>[3x]GGCGAAGAA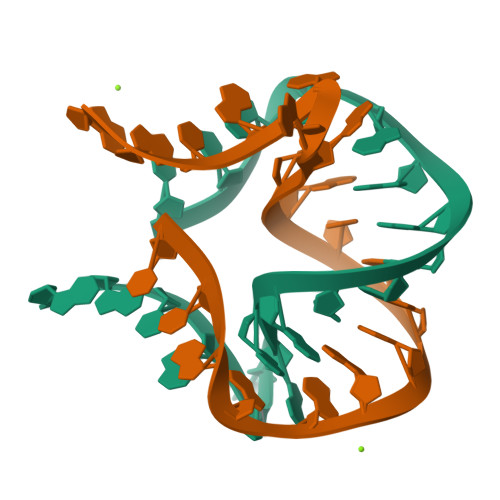CCGGGGAGCC>MKDIAIRGYCDRPSVATGETIRFYVSANETRGTFDAELVRLIHGDSNPAGPGYKEEAIKSDLEGQYPARFQRTQFGSYVEVADPDAGLQPDGAFSVHLFLWSTTPSRGRQGIASRWNDERQSGWNLAIEDGRVVFTIGDGSGATSSVVSDRPLFQQIWYSITGVYDPEKKQLRLYQKSVVNRTNSRFGLVVPLDSDCAVSADATVKAADSETSLLIAGLGEAAAQDGRTWCIAHYNGKVDAPKIYGCALGQDDAEKLSRGEIVRPISRLAHWDFSAGIGLNGIPTDHVVDASGYGHHGRCMNQPSRGSTGWNWDGHEENFIHCPEQYGALWFHEDCLDDCRWEKDFEFTVPEGLKSDFYAVKIRYEDTEDYIPFFVLPPRGTATAPILVIASTLSYLAYANEQIMHKADIGQAVAGHTPVLNENDVELHKNLSYYGLSTYDGHIDGRGVQYTSWRRPIMNLRPKHRQGFGSIWELPADLHLIDWLNHNGFEYDVATEHDLNDQGAELLRRYKVVLTGSHPAYQTWANADAWEDYLADGGRGMYLAANGMYWIVEVHPEKPWVMEVRKELGVTAWEAPPGEYHYSTNGRRGGRFRGRARATQKIWGTGMSSFGFDHSGYFVQMPDSQDERVAWIMEGIDPEERIGDGGLVGGGAGGYELDRYDLALGTPPNTLLLASSVEHSVVYTV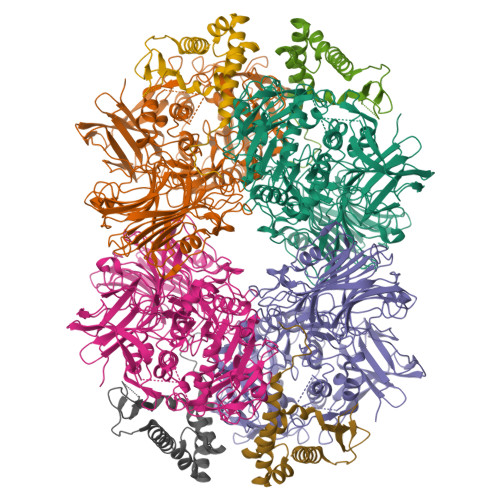IPDDKAFPHPGMNGGEHPFVRADITYFSTANGGGMFATSSISWLGSLSWNDYDNNVSKMTKNVLNQFIKDEPAPRVKLAAALEHHHHHH[4x];>MTEASESCVRDPSNYRDRSADWYAFYDERRRKEIIDIIDEHPEIVEEHAANPFGYRKHPSPYLQRVHNYFRMQPTFGRYYIYSEREWDAYRIATIREFGELPELGDERFKTEEEAMHAVFLRRIEDVRAELA[4x]> MHISDEQLKRPLRDYGEALEMWSTFQTKTQALSQSLSSQLRLILTGSGIPSKRAYQILLCVDDSSSMSDDNRSTAGNLALESLVMVARALTVLEAGQIGVMGFGTDVFVAHALTDPPFTSQDAGARVLQQFTFRQDSTDMVLLLRRTIDHFREARLIQASSSRGGEDLWQLALILSDGLV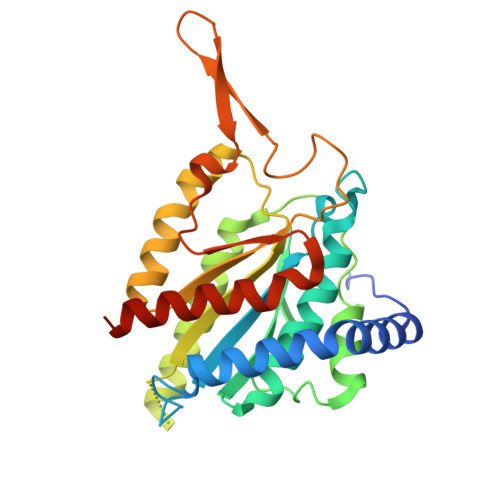QSRDHARLRPLLREAMEQRVMVVFIVMDDARSRKGHSVLELKEARFGPDGVPVIHRYLDSFPFPYYLIVHHLEDLPGALAALLRTWFAEVNSGSHHHHHH>[2x]ERAGPVTW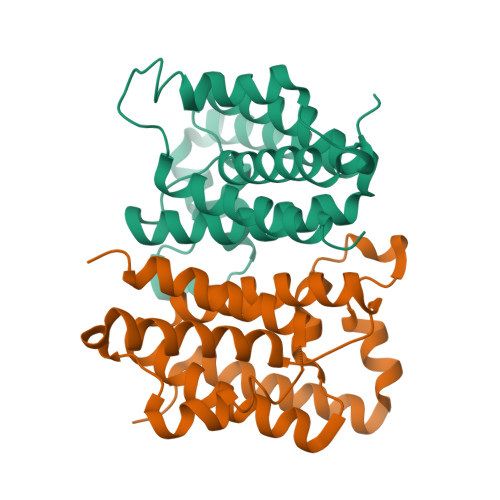VMMIACVVVFIAMQILGDQEVMLWLAWPFDPTLKFEFWRYFTHALMHFSLMHILFNLLWWWYLGGAVEKRLGSGKLIVITLISALLSGYVQQKFSGPWFGGLSGVVYALMGYVWLRGERDPQSGIYLQRGLIIFALIWIVAGWFDLFGMSMANGAHIAGLAVGLAMAFVDSLNA>ELYDKIQEAVAYVRSKTDFVPEVGLVLGSGLGPLADEVEKVAEIPYGEIPHFPVSTAPGHAGRLVLGRLEGKPVLVYKGRVHYYEGYSAEEVVFPVRVGFFLGARTFLLTSAAGGLNPRFRAGG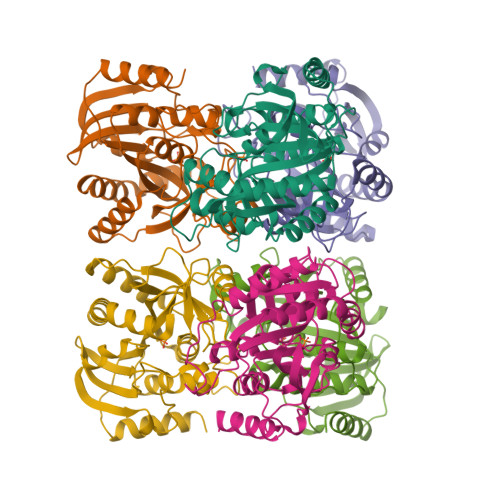IMLHLDYINFAGANPLRGPNDERLGPRFPVMFEAYDPELIELARKVARRQDLHLFEGVYAWFMGPSFASRAELRLLRELGADAIGMSTVPEVIALRHLGARVLGLSTITDMAVPEREHHATEEEVLRVAAETGPVFRRYVRGILAEL[6x]> IVGGYTCGANTVPYQVSLNSGYHFCGGSLINSQWVVSAAHCYKSGIQVRLGEDNI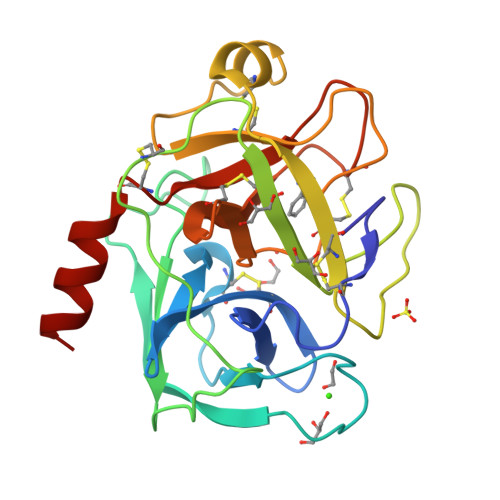NVVEGNEQFISASKSIVHPSYNSETYNNDIMLIKLKSAASLNSRVASISLPTSCASAGTQCLISGWGNTKSSGTSYPDVLKCLKAPILSDSSCKSASSFIITSNMFCAGYLEGGKDACQGDSGGPVVCSGKLQGIVSWGSGCAQKNKPGFYTKLCNYVSWIKQTIASN>[2x]SGTGSDDLKFVFVMARGGDFVAGDYAGGPKIINKEAKDSELTEQGKQEAFQLGTKLSGLYKTKLGVSKWDSKTYWPVAISQKRAQVSTLITGAGLEGDQSKRDKTWTDQELKATSFPAMESFSRFIKPSECPNYLKELLAQQGEITTIVKECISSVQQVKSKYPAVDEKMPQHIWLAYETLKKLKRQQPSSSTWMTDDLMKNLRECSAKITWLATTKTDTLRKLSGGLLLNDLFNDMDQITQGKAQPNAPGGKDSKLNVFTVSQFLVISQLAAFMPEGSKLNNKAVTASDIYPEDGSHVDIEMYQENNKWSVKLVYVSGKDKQPQTITLPGCQEKCPYEQFKSALQKYKITDEEHQKACKN

Exploration of the salivary gland composition of the rat flea, Xenopsylla cheopis, revealed several abundant acid phosphatase-like proteins whose sequences lacked one or two of their presumed catalytic residues. Our data revealed that these flea salivary acid phosphatase-like proteins have lost their expected catalytic activity and, instead, have adopted a role as scavengers of biogenic amines and leukotrienes. Additionally, XcAP-1, XcAP-2, and XcAP-3 exhibit high affinity binding to biogenic amines and leukotrienes.

The three-dimensional structure model of XcAP-1 complexed with serotonin was determined using X-ray crystallography data at a resolution of 1.75 Å. The crystal belonged to the monoclinic space group P21, and the asymmetric unit contained two near-identical XcAP-1:serotonin complexes (r.m.s.d = 0.230 Å over 356 Cα positions). In the current structure model, the serotonin molecule was found within a pocket located in the α/β-domain. The entry to the binding pocket is formed by the side chains of XcAP-1 residues Phe111, Asp227 and Asp231. Notably, both Asp227 and Asp231 form salt bridges with the protonated aliphatic amino group of serotonin, contributing to its stabilization. At the bottom of the pocket, the serotonin hydroxyl group forms hydrogen bonds with both Val8 and Asn253, while the indole nitrogen interacts with the side chain of Gln256. In XcAP-1, the residues Met9, Leu228, and Gln265 show good shape complementary with the serotonin indole group, and the pocket is closed by the Val294 residue, providing support for the serotonin molecule. Interestingly, additional interpretable electron density near the putative catalytic site of XcAP-1 was also observed, in which we modeled a palmitoleic acid molecule. The carboxyl group of the fatty acid is well defined and is oriented towards the substituted catalytic residues, while the hydrocarbon chain extends into the interior of the pocket. The fatty acid’s binding mode is predominantly shaped by the side chains of hydrophobic residues, including Ala21, Gly22, Phe120, Ile121, Leu130, Leu133, Pro166, Trp170, Leu171, Ile205, Ala209, Phe260 and Ile263.> GSTQTVHEFAKELDATNISIDKVVGAGEFGEVCSGRLKLPSKKEISVAIKTLKVGYTEKQRRDFLGEASIMGQFDHPNIIRLEGVVTKSKPVMIVTEYMENGSLDSFLRKHDAQFTVIQLVGMLRGIASGMKYLSDMGYVHRDLAARNILINSNLVCKVSDFGLSRVLEDDPEAAYTTRGGKIPIRWTSPEAIAYRKFTS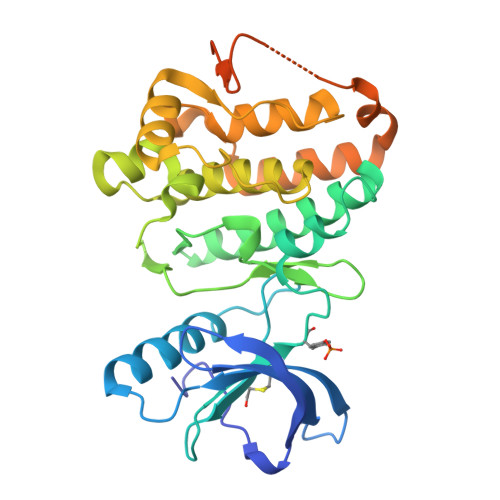ASDVWSYGIVLWEVMSYGERPYWEMSNQDVIKAVDEGYRLPPPMDCPAALYQLMLDCWQKDRNNRPKFEQIVSILDKLIRNPGSLKIITSAAARPSNLLLDQSNVDITTFRTTGDWLNGVWTAHCKEIFTGVEYSSCDTIAKIS> NKTLAAMKNFAEQYAKRTDTYFCSDLSVTAVVIEGLARHKEELGSPLCPCRHYEDKEAEVK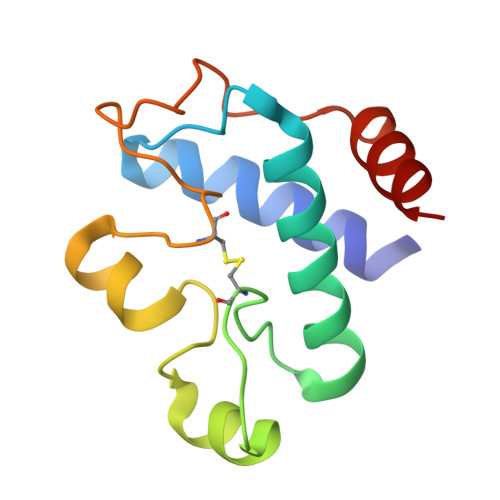NTFWNCPCVPMRERKECHCMLFLTPDNDFAGDAQDIPMETLEEVKASMA> MAHHHHHHMQKHNIKLNQNQDISQLFHDEVPLFDNSITSKDKEVIETLSEIYSIVITLDHVEKAYLKDSIDDTQYTNTVDKLLKQFKVYLNSQNKEEINKHFQSIEAFCDTYNITASNAITRLERGIPITAEHAISTTTSAPSGDNKQS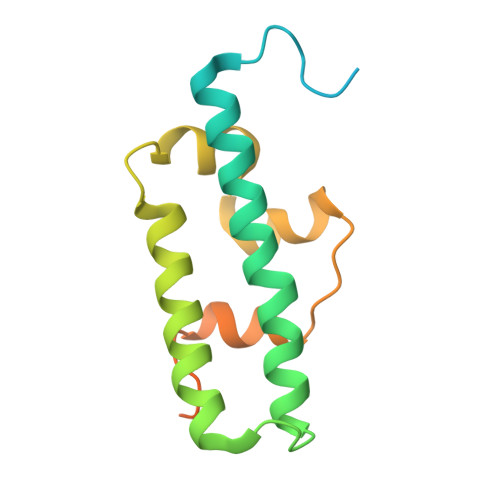SSSDKK> MGSSHHHHHHSSGLVPRGSSFEQMRQECLQRGTLFEDADFPASNSSLFYSERPQIPFVWKRPGEIVKNPEFILGGATRTDICQGELGDCWLLAAIASLTLNQKALARVIPQDQSFGPGYAGIFHFQFWQHSEWLDVVIDDRLPTFRDRLVFLHSADHNEFWSALLEKAYAKLNGSYEALKGGSAIEAMEDFTGGVAETFQTKEAPENFYEILEKALKRGSLLGCFIDTRSAAESEARTPFGLIKGHAYSVTGIDQVSFRGQRIELIRIRNPWGQVEWNGSWSDSSPEWRSVGPAEQKRLCHTALDDGE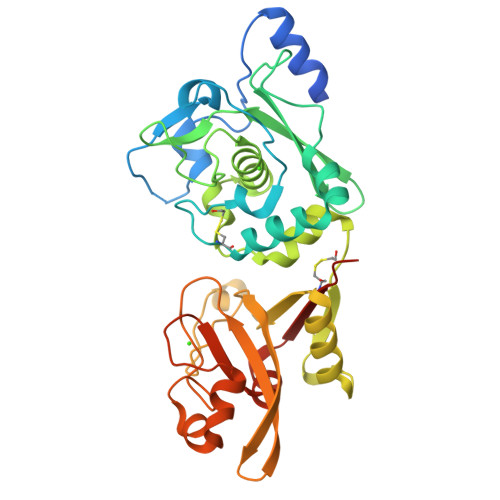FWMAFKDFKAHFDKVEICNLTPDALEEDAIH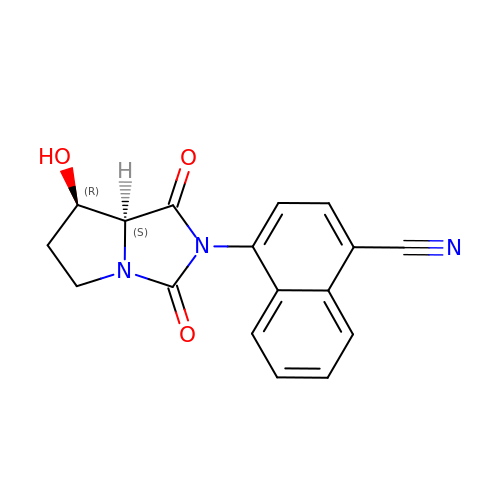4-[(7R,7AS)-7-HYDROXY-1,3-DIOXOTETRAHYDRO-1H-PYRROLO[1,2-C]IMIDAZOL-2(3H)-YL]-1-NAPHTHONITRILE | C17 H13 N3 O3 | NHBIWLQQJPSMNP-CABCVRRESA-N> AEIGGDHGYNATNIAAGQTSGAVTQIGPAVMGMVRRAIPNLIAFDICGVQPMNSPTGQVFALRAVYGKDPVAAGAKEAFHPMYGPDAMFSGQGAAKKFPALAASTQTTVGDIYTHFFQETGTVYLQASVQVTIDAGATDAAKLDAEIKKQMEAGALVEIAEGMATSIAELQEGFNGSTDNPWNEMGFRIDKQVIEAKSRQLKAAYSIELTQDLRAVHGMDADAELSGILATEIMLEINREVVDW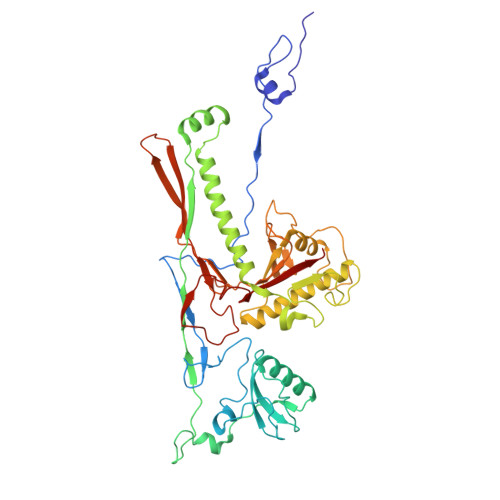INYSAQVGKSGMTLTPGSKAGVFDFQDPIDIRGARWAGESFKALLFQIDKEAVEIARQTGRGEGNFIIASRNVVNVLASVDTGISYAAQGLATGFSTDTTKSVFAGVLGGKYRVYIDQYAKQDYFTVGYKGPNEMDAGIYYAPYVALTPLRGSDPKNFQPVMGFKTRYGIGINPFAESAAQAPASRIQSGMPSILNSLGKNAYFRRVYVKGI The LMW thiol N-methyl-BSH (N-Me-BSH) has been identified in the green sulfur bacterium Chlorobaculum tepidum, revealing the presence of a putative S-adenosyl-l-methionine (SAM)-dependent methyltransferase (MT), NmbA, which could catalyze the final biosynthetic step of N-Me-BSH. In the presence of BSH and SAM, our results show that CtNmbA and PpNmbA catalyze the methylation of BSH. Our findings suggest that NmbA acts as a selective N-directed MTase of the cysteine moiety of BSH, catalyzing the last step of N-Me-BSH biosynthesis. NmbA exhibits substrate selectivity for BSH over its oxidized disulfide form, BSSB, indicating that the methylated form of BSH is likely involved in LMW thiol-dependent biochemical processes.

Overall, the structure of NmbA is organized into two domains, dominated by the canonical Class I MT Rossmann-like core domain. Across this core domain, six structural elements equivalent to the highly conserved Motifs I-VI are identified, confirming that NmbA is a SAM-binding enzyme. The active site is wedged between the Rossmann-like fold and the substrate-binding domain, with the SAM binding site located on the lower side of the cleft. The variable substrate-binding domain consists of a twisted β-sheet of four antiparallel strands, acting as a cap enclosing the active site. The Cap domain encloses the active site to form a narrow molecular basket, consequently forming a different overall structure and a tighter active site than predicted by the ab initio AlphaFold (AF) 3 model of CtNmbA. The N-terminal β'1 is directly followed by β'2, which proceeds on to α1. β'3-β′4 make up the second segment of the Cap domain (together with α'1 and an unmodelled region of 24 amino acids), following β5 of the 7BS sheet, and continuing to α5 of the C-terminal part of the protein. This Cap domain assembly results in a contorted and non-continuous four-stranded β-sheet of two subdivided segments, β'1-β′2 and β'3-β′4, where only the middle section of the β'1 and β'3 strands is connected through hydrogen bonds. Consequently, the correct organization of the β-strands according to the experimental structure results in a narrower and more rigid Cap domain, which is unlikely to undergo a conformational rearrangement upon catalysis. Structure-based docking calculations result in binding of BSH in the expected substrate binding pocket of NmbA, placing the N-atom of the BSH cysteine in proximity to the sulfonium group of SAM. The Cap domains could be rebuilt to avoid clashing between the two monomers and with a good fit to the electron density, except for residues 170–193, which did not show any electron density. PDBePISA was used to confirm that NmbA is a biological monomer, despite having two monomers in the asymmetric unit, since analysis of the protein interfaces did not reveal any specific interactions that could result in the formation of a stable quaternary structure.

>[2x]MSDHQSHSRGKNAREWFEEWFDHPLYLKVYHHRDAEEAERCVRTILDLTGIDPAWQPPHSVLDIACGAGRHALSFARTGLRVTANDLSPYLLDQARKQAKAEGINMEFSRQDMRTIRFERRFDLIAQLFSSFGYFETDQEDRDVIANIASLLNPGGWYVLDLINPVQLKSQFTPRTERNSESLSIIEERTLSERHVTKKITLHEANGRKHSFTESVRIYSPAEAFSLLESGGFAVERVVGDYEGSPFDEATSPRMMLLARLLVSRS7-[(4R,5S,6P)-7-chloro-10-[3-(4-chloro-3,5-dimethylphenoxy)propyl]-4-methyl-1-oxo-6-(1,3,5-trimethyl-1H-pyrazol-4-yl)-3,4-dihydropyrazino[1,2-a]indol-2(1H)-yl]-1-(2-methoxyethyl)-5-methyl-1H-indole-2-carboxylic 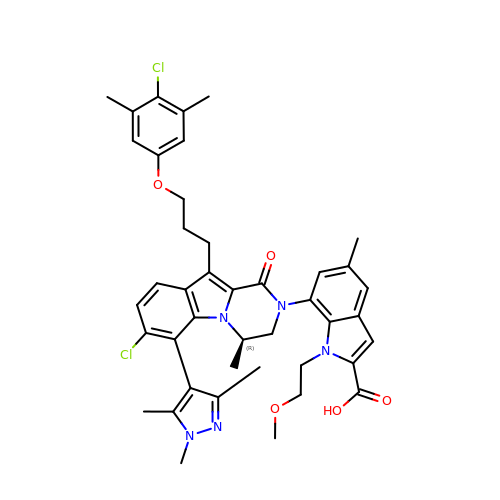acid | C42 H45 Cl2 N5 O5 | ULTJCNHXGCJYCH-RUZDIDTESA-N>[12x]MSTLKNTFFITPPDTPTQAGPENIFYDFNDGARVLLPEGKWHVRLLDADSENILFCCDVDKGWVTSSKKYFVRFRIQVFRQGEETPLLDETLKLKDRPVLISFPTGTLGALLGWFPYAERFQSLHKCRLECTMSQDIIDLLAPQYPQIQFSTPDKPRTVAPYATYRVGLYFGGDTNNQPVDFRKVGFHRSAGYILGVDPREAPVRLDLSAPRVIQEPYVCIATQSTCQAKYWNNGTGWSEVIAHLKSLGYRVMCIDRDAHYGQGFVWNHIPWGAEDFTGKLPLQERVNLLRHASFFIGLPSGLSWLAWATRIPVVLISGFSLPNSEFYTPWRVFNSHGCYGCWDDTSLNFDHHDFLWCPRHKNTDRQFECTRLITGAQVNGVINKLHRSLTEQGVEATLKKGVSNE

A subfamily of autotransporters, including AIDA-I (adhesin involved in diffuse adherence) from diffusely adhering E. coli (DAEC) 2787 and TibA from enterotoxigenic E. coli (ETEC) H10407, are glycosylated in their passenger domains, which functions in bacterial autoaggregation and adhesion to host cells. TibC catalyzes TibA/AIDA-I heptosylation and confers AIDA-I-mediated bacterial adhesion to host cells. Here we determine the crystal structures of TibC heptosyltransferase, both alone and in complex with ADP-D-glycero-β-D-manno-heptose (ADP-D,D-heptose). All the 12 TibC protomers adopt an identical structure containing an N-terminal β-barrel domain, a core catalytic domain, a β-hairpin thumb, and an iron-finger motif which are arranged into a palm-like shape.

We also crystallized the TibC dodecamer in complex with its natural ligand ADP-D-glycero-β-D-manno-heptose (ADP-D,D-heptose). This was accomplished by soaking the sugar ligand into crystals of the catalytically inactive TibC D110A mutant. ADP-D,D-heptose was convincingly modeled into each protomer and a final model of 3.88 Å was obtained. The 12 sugar ligands form an array of two parallel circles along the inner surface of the dodecamer ring and face towards the hollow center. ADP-D,D-heptose is located at the cleft between the two lobes of the catalytic domain. The adenine heterocycle fits snugly into a hydrophilic pocket and its N1 atom bears a hydrogen bond contact with Arg-286 of TibC. The hydrogen bond contact, though weak, is incompatible with a guanine due to its saturated N1, providing a structural basis for the specificity of TibC in using ADP-activated sugar donor. The β-phosphate has strong interactions with Thr-226 and Lys-230 in the ligand-binding pocket of TibC. Asp-110 is located close to the anomeric hydroxyl of heptose in the TibC–ADP-D,D-heptose complex structure. In TibC, residue 300 is a proline and its main-chain carbonyl oxygen forms two hydrogen bonds with D,D-heptose hydroxyl O4 and O6, respectively.>[2x]MTLEIFEYLEKYDYEQVVFCQDKESGLKAIIAIHDTTLGPALGGTRMWTYDSEEAAIEDALRLAKGMTYKNAAAGLNLGGAKTVIIGDPRK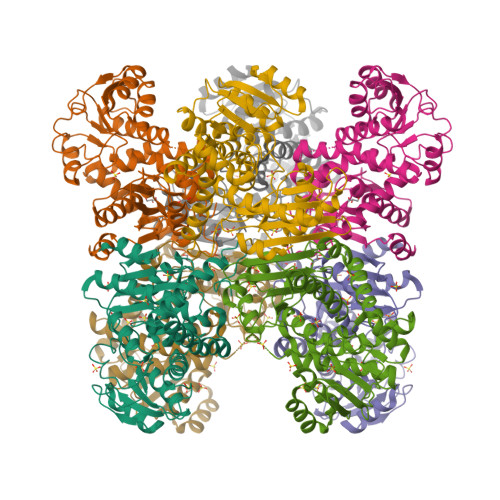DKSEAMFRALGRYIQGLNGRYITAEDVGTTVDDMDIIHEETDFVTGISPSFGSSGNPSPVTAYGVYRGMKAAAKEAVGTDNLEGKVIAVQGVGNVAYHLCKHLHAEGAKLIVTDINKEAVQRAVEEFGASAVEPNEIYGVECDIYAPCALGATVNDETIPQLKAKVIAGSANNQLKENRHGDIIHEMGIVYAPDYVINAGGVINVADELYGYNRERALKRVESIYDTIAKVIEISKRDGIATYVAADRLAEERIASLKNSRSTYLRNGHDIISRR> NLFQFGDMILQKTGKEAVHSYAIYGCYCGWGGQGRA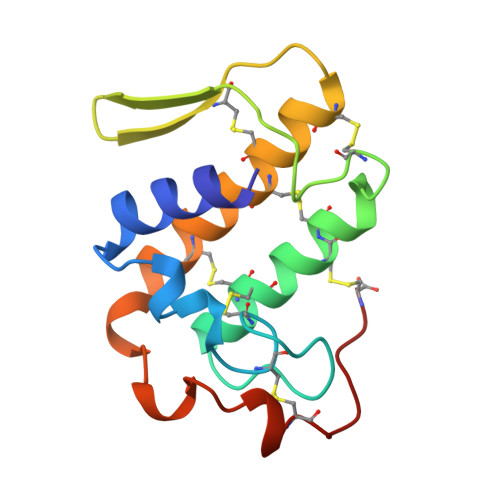QDATDRCCFAQDCCYGRVNDCNPKTATYTYSRENGDIVCGDDDLCLRAVCECDRAAAICLGENVNTYDKNYEYYSISHCTEESEQC>ACVFFCEDAAIIGLAV[4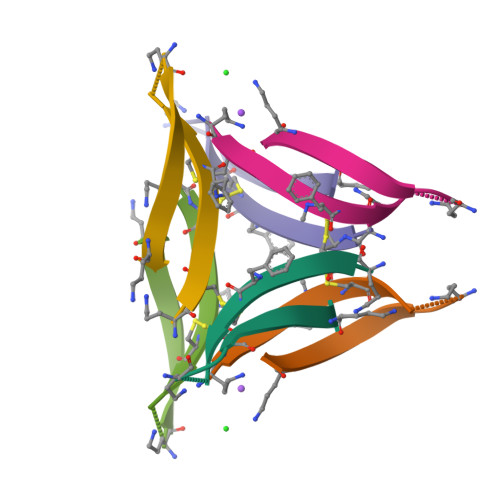x]> ADDPVYDAEGNKLVNRGKYTIVSFSDGAGIDVVATGNENPEDPLSIVKSTRNIMYATSISSEDKTPPQPRNILENMRLKINFATDPHKGDVWSVVDFQPDGQQLKL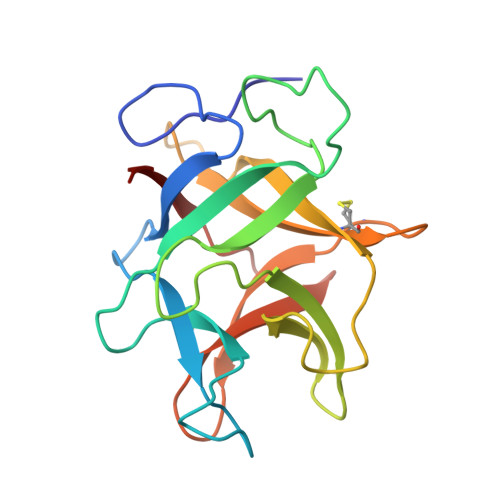AGRYPNQVKGAFTIQKGSNTPRTYKLLFCPVGSPCKNIGISTDPEGKKRLVVSYQSDPLVVKFHRHEPE>[5x]GQDMVSPPPPIADEPLTVNTGIYLIECYSLDDKAETFKVNAFLSLSWKDRRLAFDPVRSGVRVKTYEPEAIWIPEIRFVNVENARDADVVDISVSPDGTVQYLERFSARVLSPLDFRRYPFDSQTLHIYLIVRSVDTRNIVLAVDLEKVGKNDDVFLTGWDIESFTAVVKPANFALEDRLESKLDYQLRISRQYFSYIPNIILPWLFILFISWTAFWSTSYEANVTLVVS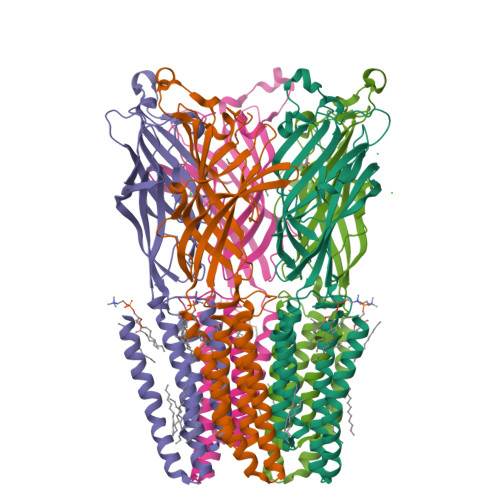TLIAHIAFNILVETNLPKTPYMTYTGAIIFMIYLFYFVAVIEVTVQHYLKVESQPARAASITRASRIAFPVVFLLANIILAFLFFGF> MAGAIIENMSTKKLCIVGGILLVFQIIAFLVGGLIAPGPTTAVSYMSVKCVDARKNHHKTKWFVPWGPNHCDKIRDIEEAIPREIEANDIVFSVHIPLPHMEMSPWFQFMLFILQLDIAFKLNNQIRENAEVSMDVSLAYRDDAFAEWTEMAHERVPRKLKCTFTSPKTPEHEGRYYECDVLPFMEIGSVAHKFYLLNIRLPVNEKKKINVGIGEIKDIRLVGIHQNGGFTKVWFAMKTFLTPSIFII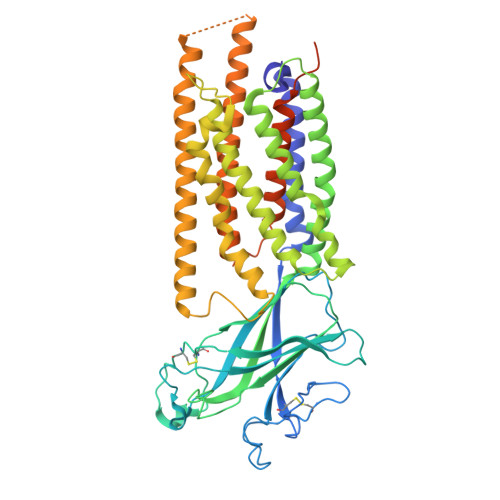MVWYWRRITMMSRPPVLLEKVIFALGISMTFINIPVEWFSIGFDWTWMLLFGDIRQGIFYAMLLSFWIIFCGEHMMDQHERNHIAGYWKQVGPIAVGSFCLFIFDMCERGVQLTNPFYSIWTTDIGTELAMAFIIVAGICLCLYFLFLCFMVFQVFRNISGKQSSLPAMSKVRRLHYEGLIFRFKFLMLITLACAAMTVIFFIVSQVTEGHWKWGGVTVQVNSAFFTGIYGMWNLYVFALMFLYAPSHKNYGEDQSNGDLGVHSGEELQLTTTITHVDGPTEIYKLTRKEAQE> TDIENVPAKIVLKADKQKDMKDYIDDLRTYNNSYSNVVTVAGEDRIETAIELSYKYYNSDDDNAVTDIAADNVVLVGSQAIVDGLVASPLASEKHAPLLLTSKDKLDSSVKSEIKRVMDLKTTSGINTSKKVYLAGGVNSISKDVENELKDMGVKVVRLAGDDRYETSLAIADEVGLDNDKAFVVGGTGLADAMSIAPVASQLKDSNGNMDVVDGDATPIVVVDGKAKDINAATEDFLDNAQVDIIGGENSVSKDIEEAIDDATGKEPNRTSGDDRQDTNAEVMKETDYFEKASVENYFVAKDGSTKEDQLVDALAAAPVAA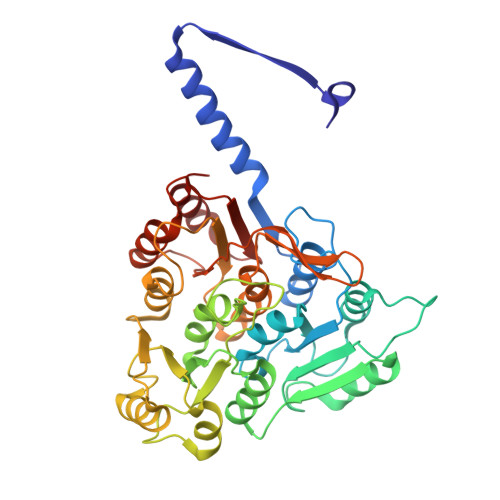NFGATYTKNGSTYTKSGNVSPAPIVLATDTLSGDQNVGVSKSVSDDGGKNLVQVGKGIASSVISKMKDLLDM>MDVRTLAVGKAHLEALLATRKMTLEHLQDVRHDATQVYFDGLEHLQNVAQYLAIPLSEFFVGQTQSDLDDGVKIARRNGGFKREEIRGGVHYYTYEHLVTTNQDPGLMALRLDLHSDDEQPLRLNGGHGSREIVYVTRGAVRVRWVGDNDELKEDVLNEGDSIFILPNVPHSFTNHVGGAKSEIIAI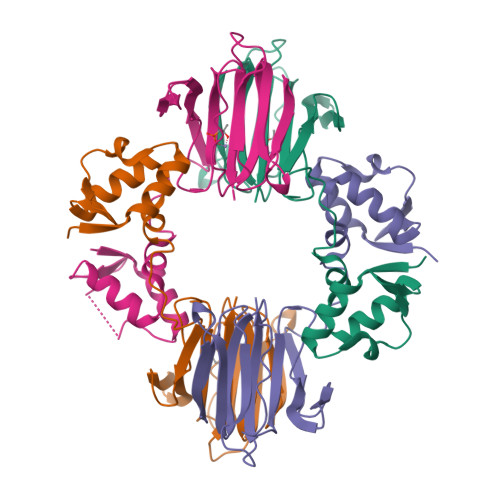NYG[4x]YggS is a PLP-binding protein found in bacteria and humans that mediates PLP homeostasis by delivering PLP to target enzymes or by performing a protective function. Here, we report a functional and structural analysis of YggS from Fusobacterium nucleatum (FnYggS). FnYggS consists of 8 β-strands and 10 α-helices and forms a TIM barrel fold typical of the type III fold of PLP-dependent enzymes. Although FnYggS exhibited low (<35%) amino acid sequence similarity with previously studied YggS proteins, its overall structure and PLP-binding site were highly conserved.

To better understand the properties underlying PLP recognition, we determined the crystal structure of FnYggS at 2.08 Å resolution by Se-SAD. The crystal structure belonged to the monoclinic space group P21 with a = 37.929 Å, b = 146.375 Å, c = 74.128 Å, α = γ = 90° and β = 93.355°. The electron density map showed a clear electron density for all of the amino acid residues from Met1 to Lys223 in the A chain and C chain, while in the B chain of FnYggS, most amino acid residues from Met1 to Lys223 showed a clear electron density, except for Glu128-Gln132. The crystal structure of FnYggS-SeMet did not exhibit the electron density considered to represent the PLP molecule, consistent with our spectroscopy experiments showing the absence of PLP binding in FnYggS-SeMet. Instead, a sulfate ion was observed in the PLP-binding site of FnYggS. This sulfate ion was coordinated by the hydroxyl oxygen atom of Ser201 (2.7 Å), the nitrogen atom of Ser201 (3.0 Å), the nitrogen atom of Gly218 (2.8 Å), and the nitrogen atom of Thr219 (2.9 Å). Interestingly, the position of the sulfate ion in FnYggS-SeMet was almost the same as that of the phosphate group of PLP in the EcYggS structure. This result indicates that the sulfate ion in FnYggS-SeMet is positioned to provide the binding moiety, as is the phosphate group in PLP. FnYggS contains seven methionine residues, among which Met200 is located at the PLP-binding site and is downstream of Ser201, which is involved in PLP binding. During structural refinement, the side chain of SeMet200 showed two distinct conformations.

>MSIKTNVEEILEDIKKYSPYPEKVKLVAVTKYSSVEDIEKFLETGQNICGENKVQVIKDKIEYFKEKNKKIKWHFIGNLQKNKVKYIIDDVDLIHSVNKLSLAQEINKKAEQSSKIMDVLLEINVYGEESKQGYSLDELKCDIIELQNLKNLNIIGVMTMAPFTDDEKILRMVFSELRKIKDELNKEYFNNNLTELSMGMSNDYKIALQEGSTFIRVGTKIFK[3x]>[2x]TIQPGTGYNNGYFYSYWNDGHGGVTYTNGPGGQFSVNWSNSGDFVGGKGWQPGTKNKVINFSGSYNPNGNSYLSVYGWSRNPLIEYYIVENFGTYNPSTGATKLGEVTSDGSVYDIYR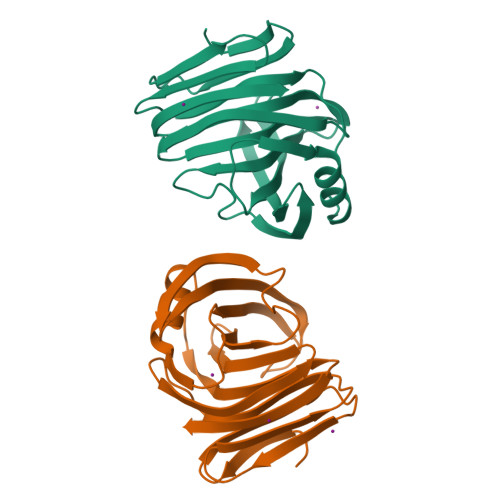TQRVNQPSIIGTATFYQYWSVRRNHRSSGSVNTANHFNAWAQQGLTLGTMDYQIVAVEGYFSSGSASITVS>MISPNLTANVEIDGKQYNTFTEPPKALAGERAKVKFPIKDMTEFLHGGEENVTMIERLMTELERDPVLNVSGDYDMPKEQLRETAVARIAALSGHWKKDTEKEALLRSQLHGIVDMGTRIRLGVHTGLFMGAIRGSGTKEQYDYWVRKGAADVKGFYGCFAMTELGHGSNVAGLETTATYIQDTDEFIINTPNTGATKWWIGGAAHSATHTACFARLLVDGKDYGVKIFVVQLRDVSSHSLMPGIALGDIGKKMGRDAIDNGWIQFTNVRIPRQNMLMKYAKVSSTGKVSQPPLAQLTYGALIGGRVTMI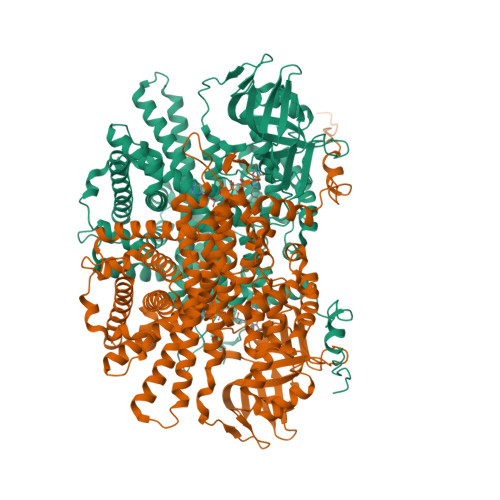ADSFFVSQRFITIALRYACVRRQFGTTPGQPETKIIDYPYHQRRLLPLLAFTYAMKMAADQSQIQYDQTTDLLQTIDPKDKGALGKAIVDLKELFASSAGLKAFTTWTCANIIDQCRQACGGHGYSGYNGFGQAYADWVVQCTWEGDNNVLCLSMGRGLIQSCLGHRKGKPLGSSVGYLANKGLEQATLSGRDLKDPKVLIEAWEKVANGAIQRATDKFVELTKGGLSPDQAFEELSQQRFQCAKIHTRKHLVTAFYERINASAKADVKPYLINLANLFTLWSIEEDSGLFLREGFLQPKDIDQVTELVNHYCKEVRDQVAGYTDAFGLSDWFINAPIGNYDGDVYKHYFAKVNQQNPAQNPRPPYYESTLRPFLFREDEDDDICELDEELEHHHHHH[2x]> SMSVRPPVLVDIKFNPEGVDRVLKTAFADRGSINLADPANRERDFSETEYALLWKPDADLFRRAPNLKVIFSGGAGVDHIIGMAGLPDIPIVRFVDRSLTTRMSEWVVMQCLMHLRGQYGHDSHQRRREWAKLIAPEAAEVTVGVMGLGILGQDAVAKLKVMGFNVIGWSRTRKTIEGVETFDAGELDRFLA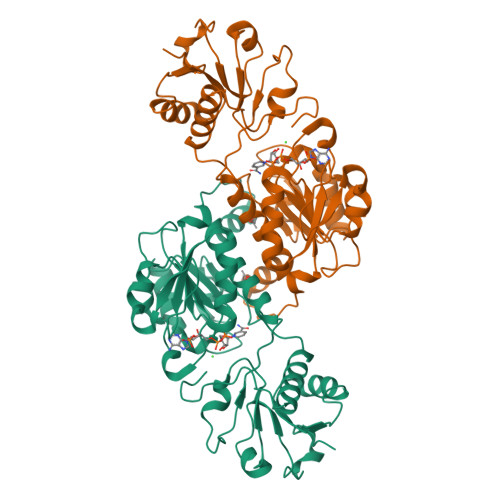KTDILVGLLPLTPETTGFYDSELFKKLRRDGALGQPVFINAGRGKSQIETDIVSAVREGTLGGASLDVFEVEPLATDSPLWELENVFITPHDAAVSEENALFRHVEMQIARFERGEPLQFVIDRAAGY> ATPSTLAELCTDSIVKAALPPSEFIQGITIDSDSVTTEVVTNSSVSSEFYPSATINYCNVTFAYSHDGIDGDQVLLEIWLPAPTDFQNRWLSTGGGGYAINSGDQSLPGGVMYGAASGMTDGGFGGFSNNADTAMLLANGTLDYETLYMFAYKAHRELSLIGKALTRNVYGMSDSDKLYAYYQGCSEGGREGWSQVQRFGDEWDGAIIGAPAFRWSFQQTQHLYSNVVEKTLDYYPPPCELDKIVNETIAACDAMDGKVDWVVARTDLCLLDFDISTIEGKPYSCAASRGTPAQNGTVSAKGIEVAKTIINGLHDSQGRRVYFSYQPTAAFDDAETQYNSTTGQWGLDIDQLGGEYIALLVDKNGTTLDSLDGVTYDTLKDWMISGLQEYYSTLQTTWPDLTPFHEAGGKVIHFHGDADFSIPTAASIRYWESVRSIMYPNQDYNSSAEALNEWYRLYTVPGAGH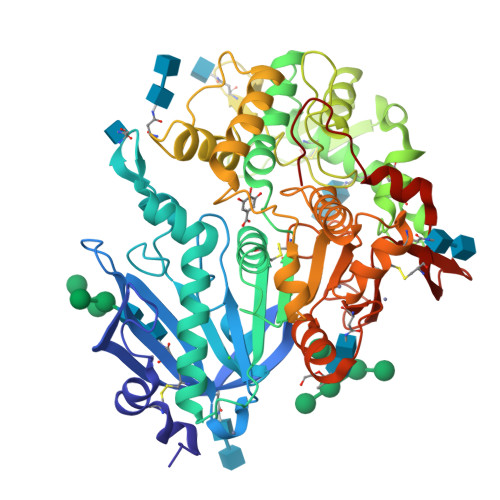CATNDAMPNGPFPQTNMAVMIDWVENGVVPTTLNATVLQGENEGQNQQLCAWPLRPLWTNNGTTMECVYNQRSIDSWHYDLDAVPMPVY> GSHMGNDIEYYT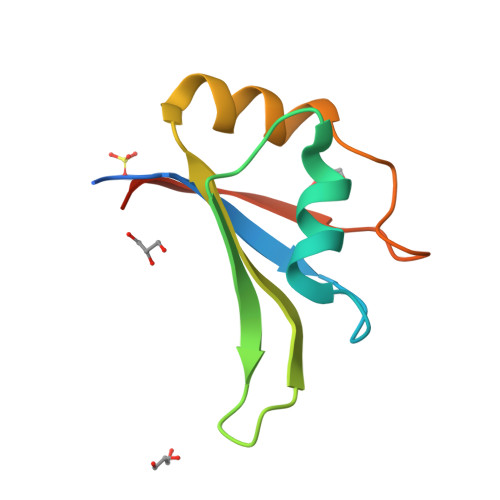IHMRGLPYTSFENDVFKFFEPIRPANVRINYNKKGLHSGTADAYFDTYEDSQVAMKRHREQMGSRYIELFYDGKTRGLNG> GSHMASDPLLSVLMWGVNHSINELSHVQIPVM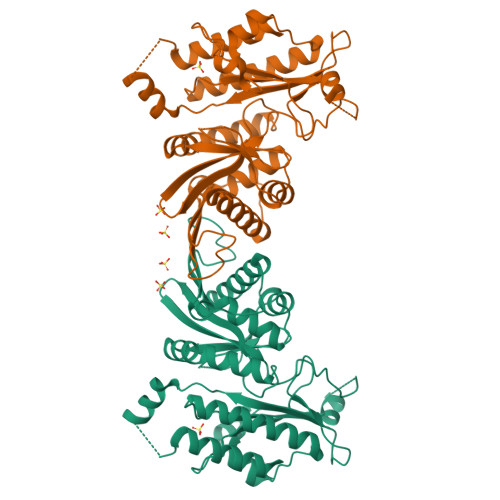LMPDDFKAYSKIKVDNHLFNKENMPSHFKFKEYCPMVFRNLRERFGIDDQDFQNSLTRSAPLPNDSQARSGARFHTSYDKRYIIKTITSEDVAEMHNILKKYHQYIVECHGITLLPQFLGMYRLNVDGVEIYVIVTRNVFSHRLSVYRKYDLKGSTVAREASDKEKAKELPTLKDNDFINEGQKIYIDDNNKKVFLEKLKKDVEFLAQLKLMDYSLLVGIHDVERAEQEEVECEENDGEEEGESDGTHPVGTPPDSPGNTLNSSPPLAPGEFDPNIDVYGIKCHENSPRKEVYFMAIIDILTHYDAKKKAAHAAKTVKHGAGAEISTVNPEQYSKRFLDFIGHIL> YILPSFIEHSSFGVKESNPYNKLFEERIIFLGVQVDDASANDIMAQLLVLESLDPDRDITMYINSPGGGFTSLMAIYDTMQYVRADIQTVCLGQAASAAAVLLAAGTPGKRMALPNARVLIHQPSLSGVIQGQFSD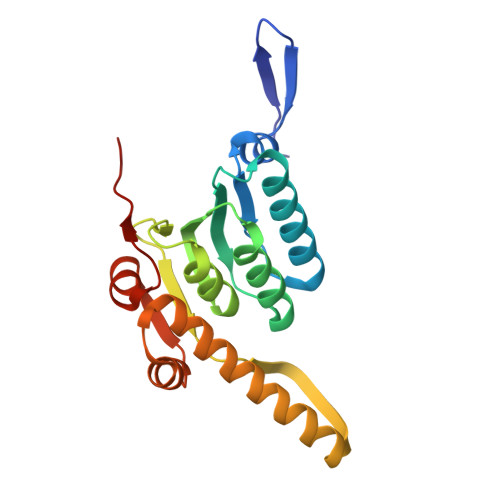LEIQAAEIERMRTLMETTLARHTGKDAGVIRKDTDRDKILTAEEAKDYGIIDTVLEYRKLS>MNYKELEKMLDVIFENSEIKEIDLFFDPEVEISKQEFEDLVKNADPLQKVVGDNYITETFEWWEFENQYLEFELD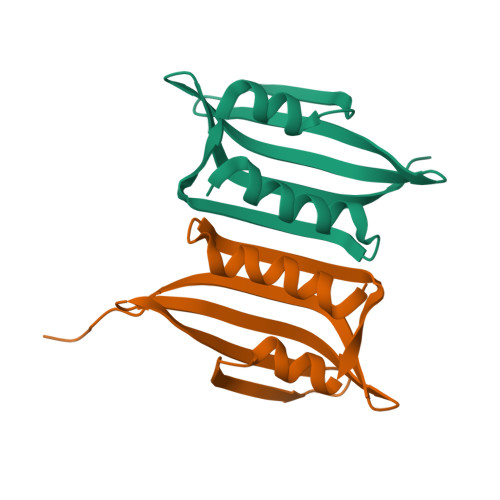YYVKDEKIFVLEMHFWRKIRKLEHHHHHH[6x]4-BROMO-2,6-DICHLORO-N-(1,3,5-TRIMETHYL-1H-PYRAZOL-4-YL)BENZENESULFONAMIDE 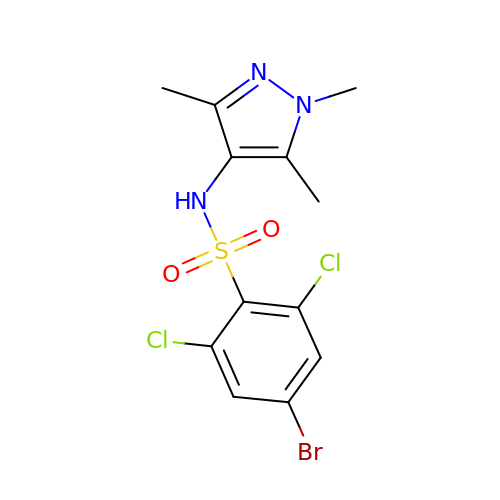| C12 H12 Br Cl2 N3 O2 S | SXCJBRNVTQTKSN-UHFFFAOYSA-N>[2x]MSTTQTPDLDAIVIGAGFGGIYMLHKLRNDLGLSVRVFEKGGGVGGTWYWNKYPGAKSDTEGFVYRYSFDKELLREYDWTTRYLDQPDVLAYLEHVVERYDLARDIQLNTEVTDAIFDEETELWRVTTAGGETLTARFLVTALGLLSRSNIPDIPGRDSFAGRLVHTNAWPEDLDITGKRVGVIGTGSTGTQFIVAAAKMAEQLTVFQRTPQYCVPSGNGPMDPDEVARIKQNFDSIWDQVRSSTVAFGFEESTVEAMSVSESERQRVFQQAWDKGNGFRFMFGTFCDIATNPEAN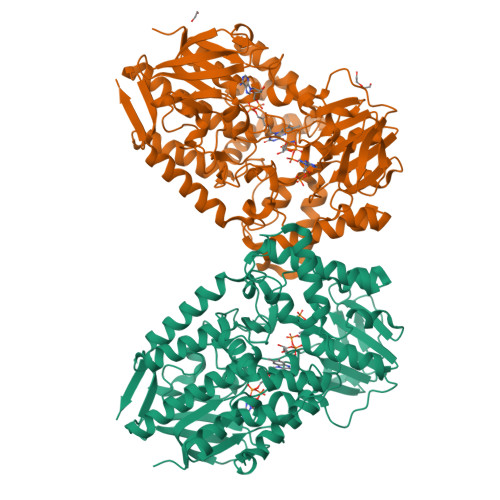AAAAAFIRSKIAEIVKDPETARKLTPTDLYAKRPLCNEGYYETYNRDNVSLVSLKETPIEEIVPQGVRTSDGVVHELDVLVFATGFDAVDGNYRAMNLRGRDGRHINEHWTEGPTSYLGVTKAGFPNMFMILGPNGPFTNTPPSIEAQVEWISDLIDKATREGLTTVEPTADAEREWTETCAEIANMTLFPKADSWIFGANIPGKRHAVMFYLGGLGNYRRQLADVADGGYRGFQLRGERAQAVA>GPHMAAQKTELEQHEALLHQARQYRQQTKARQQWLEEMQHDYSGFVQGVKEVLKARDLLPGIHGAIVELIRVPDRYETAIETALGGAMQHIVVDSEQAARQAIHYLKTNGYGRATFLPLDVIKARALSERERAAIDRHPAFVGIASELVEYDRAYRAAIAHLLGHVIVTADLKGANELAKLLHYRYRLVTLDGDVVSPGGAMTGGGAAKKTASLLSRNRELEMLSAKLQEMDETIARLERAVAAKRHELAEQEAQAA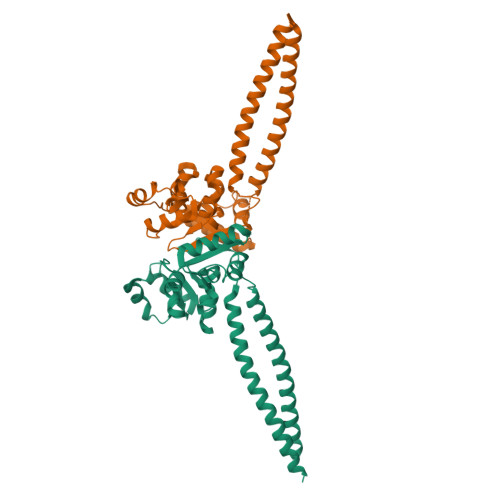ALQE[2x]> MPGSAAKGSELSERIESFVETLKRGGGPRSSEEMARETLGLLRQIITDHRWSNAGELMELIRREGRRMTAAQPSETTVGNMVRRVLKIIREEYGRLHGRSDESDQQESLHKLLTSGGLNEDFSFHYAQLQSNIIEAINELLVELEGTMENIAAQALEHIDSNEVIMTIGFSRTVEAFLKEAAR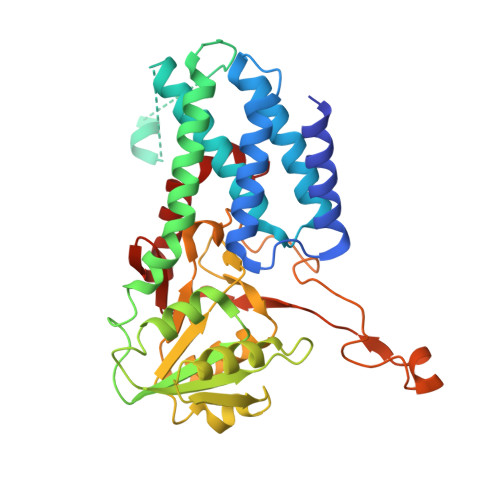KRKFHVIVAECAPFCQGHEMAVNLSKAGIETTVMTDAAIFAVMSRVNKVIIGTKTILANGALRAVTGTHTLALAAKHHSTPLIVCAPMFKLSPQFPNEEDSFHKFVAPEEVLPFTEGDILEKVSVHCPVFDYVPPELITLFISNIGGNAPSYIYRLMSELYHPDDHVL> PNSMKNIESLFDYSAGQFEFIDHLLTMGVGVHFAALIFFLVVSQFVAPKYRIATALSCIVMVSAGLILNSQAVMWTDAYAYVDGSYQLQDLTFSNGYRYVNWMANIPCLLLQLLIVLNLKGKELFSTATWLILAAWGMIITGYVGQLYEVDDIAQLMIWGAVSTAFFVVMNWIVGTKIFKNRATMLGGTDSTITKVFWLMMFAWTLYPIAYLVPAFMNNADGVVLRQLLFTIADISSKVIYGLMITYIAIQQSAAAGYVPAQQALGRIGMDSKAA

In contrast, the NTQ rhodopsin functions as a light-driven inward chloride pump (called ClR). Here we report the atomic crystal structure of ClR from the flavobacterium Nonlabens marinus S1-08T. The structure reveals two chloride ion-binding sites, one at the active centre of the pump and the other on a loop in the cytoplasmic side, suggesting the pathway of chloride ion movement in ClR. The ClR structure comprises a short N-terminal helix, seven transmembrane helices (TM A–TM G), a C-terminal helix and three loops connecting the transmembrane helices on both extracellular and cytosolic sides.

Because Asn98 and Thr102 are the only residues of ClR directly interacting with Cl−-I, we investigated whether the interaction between Asn98 or Thr102 and Cl−-I is essential for the chloride-pumping activity of ClR. We expressed several ClR mutants (N98A, N98D and N98L for Asn98; and T102D, T102N and T102V for Thr102) in Escherichia coli cells. In most mutants, except T102N, the chloride-pumping activities were eliminated or substantially decreased (<50% of the wild-type ClR), indicating that Asn98 and Thr102 play significant roles in chloride pumping. Of the mutants, T102N retained ∼70% of its pumping activity compared with the wild-type protein, whereas T102D completely lost its pumping activity. T102N's absorption spectra showed a blue shift in 1.5 M NaCl (λmax from 562 to 529 nm) suggesting that a chloride ion can bind at PSB but T102D's absorption spectra did not change in 1.5 M NaCl. We crystallized T102N and T102D proteins and collected diffraction data. The T102N crystal structure shows that ND-1 of the mutated Asn is hydrogen-bonded to Cl−-I, as is OG-1 of Thr102 in the wild type. Taken together, these results show that the direct hydrogen bond between Asn98/Thr102 (Asn98 and Thr102) and Cl−-I is crucial for the binding of Cl−-I, as well as for the chloride-pumping activity of ClR.>[2x]MLGLKTSIIGRRVIYFQEITSTNEFAKTSYLEEGTVIVADKQTMGHGRLNRKWESPEGGLWLSIVLSPKVPQKDLPKIVFLGAVGVVETLKEFSIDGRIKWPNAVL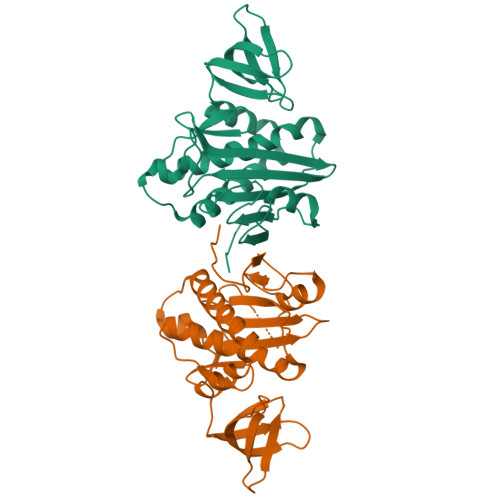VNYKKIAGVLVEGKGDKIVLGIGLNVNNKVPNGATSMKLELGSEVPLLSVFRSLITNLDRLYLNFLKNPMDILNLVRDNMILGVRVKILGDGSFEGIAEDIDDFGRLIIRLDSGEVKKVIYGDVSLRFL> GSAMGSSSVAISKPLLKLKLLDALRQGSFPNLQDLLKKQFQPLDDPNVQQVLHLMLHYAVQVAPMAVIKEIVHHWVSTTNTTFLNIHLDL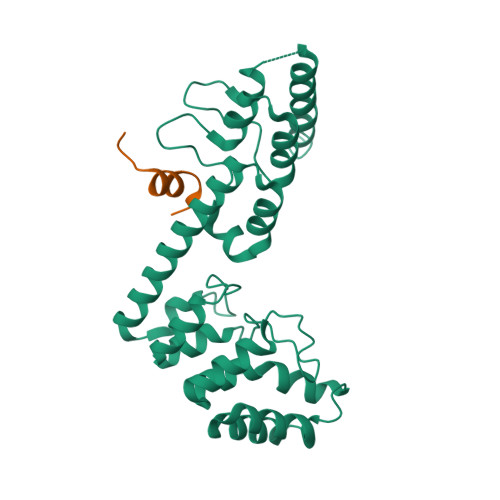NERDSNGNTPLHIAAYQSRGDIVAFLLDQPTINDCVLNNSHLQAIEMCKNLNIAQMMQVKRSTYVAETAQEFRTAFNNRDFGHLESILSSPRNAELLDINGMDPETGDTVLHEFVKKRDVIMCRWLLEHGADPFKRDRKGKLPIELVRKVNENDTATNTKIAIDIELKKLLERATREQSVIDVT;> KHYNDGERAVLQFGKNRSEPIILSYKD> MKKFNIKSLTLLIVLLPLIVNANNIDSHLLEQNDIAKYVAQSDTVGSFFE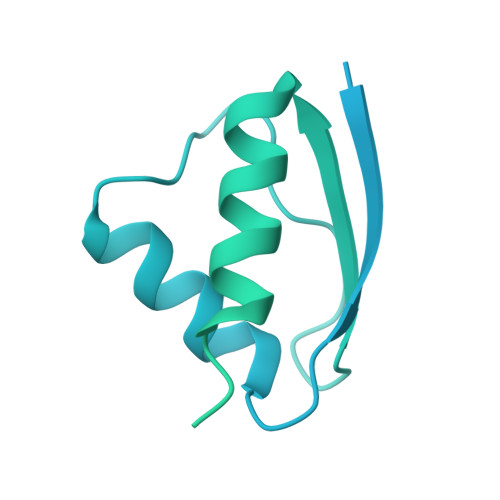RFSALLNYPIVVSKQAAKKRISGEFDLSNPEEMLEKLTLLVGLIWYKDGNALYIYDSGELISKVILLENISLNYLIQYLKDANLYDHRYPIRGNISDKTFYISGPPALVELVANTATLLDKQVSSIGTDKVNFGVIKLKNTFVSDRTYNMRGEDIVIPGVATVVERLLNNGKALSNRQAQNDPMPPFNITQKVSEDSNDFSFSSVTNSSILEDVSLIAYPETNSILVKGNDQQIQIIRDIITQLDVAKRHIELSLWIIDIDKSELNNLGVNWQGTASFGDSFGASFNMSSSASISTLDGNKFIASVMALNQKKKANVVSRPVILTQENIPAIFDNNRTFYVSLVGERNSSLEHVTYGTLINVIPRFSSRGQIEMSLTIEDGTGNSQSNYNYNNENTSVLPEVGRTKISTIARVPQGKSLLIGGYTHETNSNEIISIPFLSSIPVIGNVFKYKTSNISNIVRVFLIQPREIKESSYYNTAEYKSLISEREIQKTTQIIPSETTLLEDEKSLVSYLNY>MWSHPQFEKTTNAGPLHPYWPQHLRLDNFVPNDRPTWHILAGLFSVTGVLVVTTWLLSGRAAVVPLGTWRRLSLCWFAVCGFIHLVIEGWFVLYYEDLLGDQAFLSQLWKEYAKGDSRYILGDNFTVCMETITACLWGPLSLWVVIAFLRQHPLRFILQLVVSVGQIYGDVLYFLTEHRDGFQHGELGHPLYFWFYFV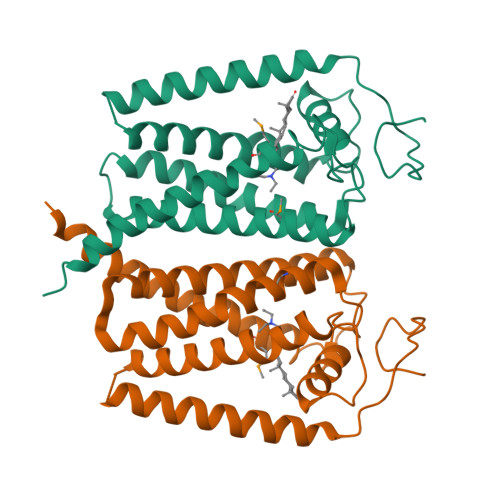FMNALWLVLPGVLVLDAVKHLTHAQSTLDAKATKAKSKKN[3x]>MNGEAICSALPTIPYHKLADLRYLSRGASGTVSSARHADWRVQVAVKHLHIHTPLLDSERKDVLREAEILHKARF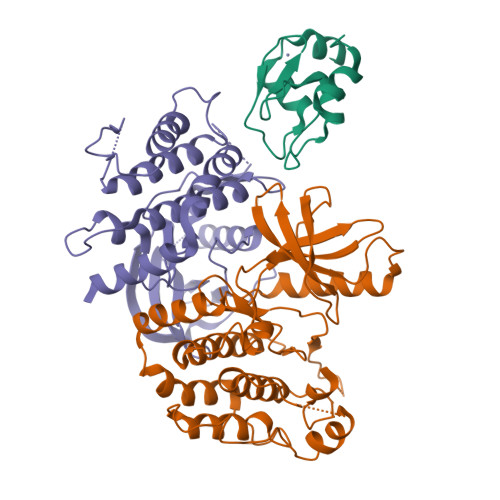SYILPILGICNEPEFLGIVTEYMPNGSLNELLHRKTEYPDVAWPLRFRILHEIALGVNYLHNMTPPLLHHDLKTQNILLDNEFHVKIADFGLSKWRMMSLSQSRSSKSAPEGGTIIYMPPENYEPGQKSRASIKHDIYSYAVITWEVLSRKQPFEDVTNPLQIMYSVSQGHRPVINEESLPYDIPHRARMISLIESGWAQNPDERPSFLKCLIELEPVLRTFEEITFLEAVIQLKKTKLQSV[2x];> YPRNPAMYSEEARLKSFQNWPDYAHLTPRELASAGLYYTGIGDQVQCFCCGGKLKNWEPCDRAWSEHRRHFPNCFFVLGRNLNIRSE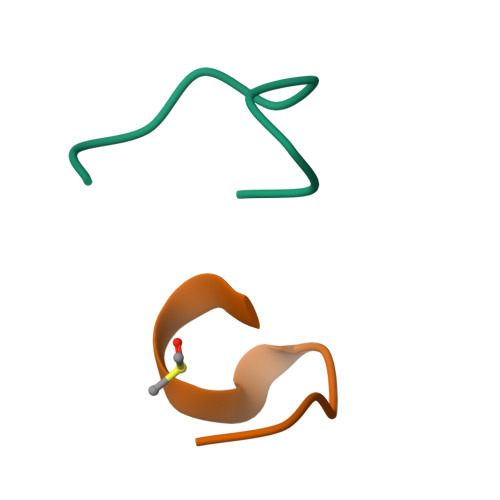>[2x]AFGKVFPQAG>GSHMAVHLTRIYTRTGDDGTTGLSDMSRVAKTDARLVAYADCDEANAAIGAALALGHPDTQITDVLRQIQNDLFDAGADLSTPIVENPKHPPLRIAQSYIDRLEGWCDAYNAGLPALKSFVLPGGSPLSALL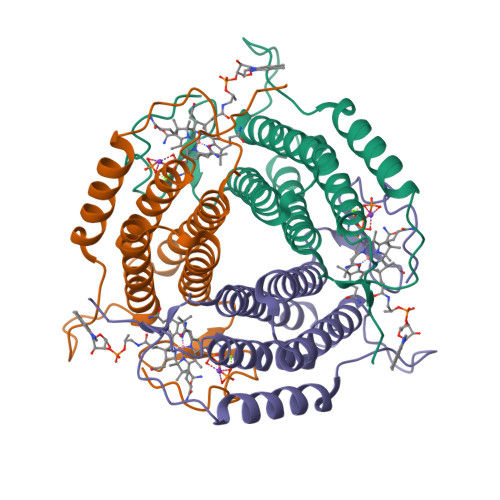HVARTVVRRAERSAWAAVDAHPEGVSVLPAKYLNRLSDLLFILSRVANPDGDVLWRPGGDRTAS[3x]Signal transduction by these ligands requires type I and type II transmembrane receptor serine/threonine kinases which form heterotetrameric complexes for ligand interaction. Type I receptors phosphorylate SMAD family transcription factors, whereas type II receptors are required to activate the type I receptors by phosphorylation of their juxtamembrane GS (glycine-serine rich) domain. Type I receptors ALK1/ACVRL1, ALK2/ACVR1, ALK3/BMPR1A and ALK6/BMPR1B all participate in BMP signalling and phosphorylate SMAD1/5/8. By contrast, fibrodysplasia ossificans progressiva (FOP) is a rare monogenic condition in which a gain of function germline mutation in ACVR1 leads to increased signalling through ALK2 in response to BMP ligands as well as neofunction in response to Activin A and the consequent formation of heterotopic bone in muscle and connective tissue.

Here we determined the crystal structure of ALK2 in complex with LDN-212854 revealing subtle differences in its binding compared to LDN-193189. Four protein-inhibitor complexes were observed in the asymmetric unit with no significant structural differences. The structure of the ALK2 kinase domain in complex with LDN-212854 was observed to adopt an inactive conformation similar to the more complete structure of the ALK2 GS and kinase domains bound to FKBP12. In this shared inhibitory conformation there is close packing of the kinase N and C-lobes creating strong interactions for the inhibitor bound in the central ATP-binding pocket. However, at the solvent-exposed entrance of the active site the binding of ATP and substrate would be sterically occluded by the inward folding of the activation segment. Here, a single hydrogen bond is observed between the N-1 nitrogen of the pyrazolo[1,5-a]pyrimidine moiety and the backbone nitrogen of His286. Most importantly, the central pyrazolo[1,5-a]pyrimidine moiety orients the 5-quinoline group to the back pocket where it packs below Val222. In the inactive ALK2 conformation the catalytically important salt bridge between Lys235 (β3 strand) and Glu248 (αC) is broken and these side chains are free for interaction with inhibitors. The nitrogen of the 5-quinoline of LDN-212854 appears optimally positioned to form a water-mediated hydrogen bond that bifurcates to contact both Lys235 and Glu248. Thus, the 5-quinoline of LDN-212854 appears particularly favourable for establishing a larger network of water-mediated hydrogen bonding in ALK2.

>[4x]SMQRTVARDITLLECVGKGRYGEVWRGSWQGENVAVKIFSSRDEKSWFRETELYNTVMLRHENILGFIASDMTSRHSSTQLWLITHYHEMGSLYDYLQLTTLDTVSCLRIVLSIASGLAHLHIEIFGTQGKPAIAHRDLKSKNILVKKNGQCCIADLGLAVMHSQSTNQLDVGNNPRVGTKRYMAPEVLDETIQVDCFDSYKRVDIWAFGLVLWEVARRMVSNGIVEDYKPPFYDVVPNDPSFEDMRKVVCVDQQRPNIPNRWFSDPTLTSLAKLMKECWYQNPSARLTALRIKKTLTKID> AQSVPYGVSQIKAPALHSQGYTGSNVKVAVIDSGIDSSHPDLKVAGGASMVPSETNPFQDNNSHGTHVAGTVAALNNSIGVLGVAPSASLYAVKVLGADGSGQYSWIINGIEWAIANNMDVINMSLGGPSGSAALKAAVDKAVASGVVVVAAAGNEGTSGSSSTVGYPGKYPSVIAVGAVDSSNQRASFSSVGPELDVMAPGVSIQSTLPGNKYGAYNGTSMASPHVAGAAALILSKHPNWTNTQVRSSLENTTTKLGDSFYYGKGLINVQAAAQ;> YAP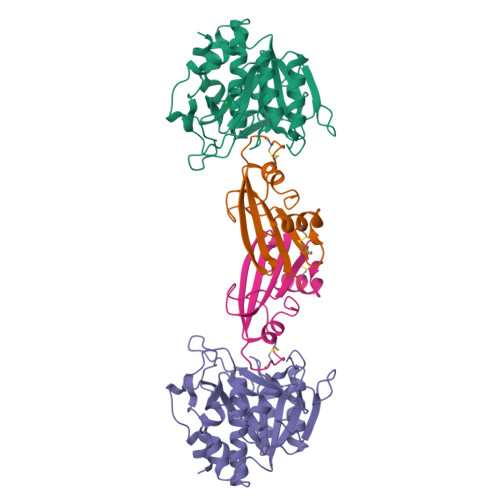SALVLTVGKGVSATTAAPERAVTLTCAPGPSGTHPAAGSACADLAAVGGDLNALTRGEDVGCPKVYDPVLLTVDGVWQGKRVSYERVFSNECEMNAHGSSVFAF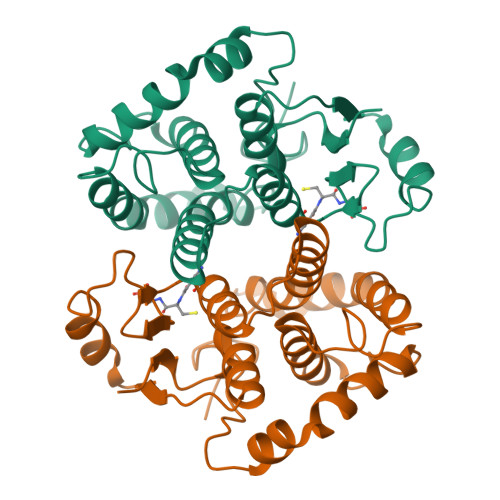> MSPILGYWKIKGLVQPTRLLLEYLEEKYEEHLYERDEGDKWRNKKFELGCEFPNLPYYIDGDVKLTQSMAIIRYIADKHNMLGGCPKERAEISMLEGAVLDIRYGVSRIAYSKDFETLKVDFLSKLPEMLKMFEDRLCHKTYLNGDHVTHPDFMLYDALDVVLYMDPMCLDAFPKLVCFKKRIEAIPQIDKYLKSSKYIAWPLQGWQATFGGGD> KASFTDEEDEFILDVVRKNPTRRTTHTLYDEISHYVPNHTGNSIRHRFRVYLSKRLEYVYEVDKFGKLVRDDDGNLIKTKVLPPSIKRKFSADEDYTLAIAVKKQFYRDLFQIDPDTGRSLITDEDTPTAIARRNMTMDPNHVPGSEPNFA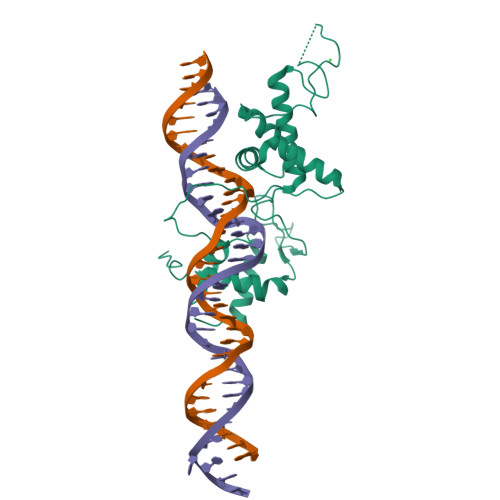AYRTQSRRGPIAREFFKHFAEEHAAHTENAWRDRFRKFLLAYGIDDYISYYEAEKAQNREPEPMKNLTNRPKRPGVPTPGNYNSAAKRARN> APLADYKDDDDKLAGTPSVDHGFLVTRHSQTIDDPQCPSGTKILYHGYSLLYVQGNERAHGQDLGTAGSCLRKFSTMPFLFCNINNVCNFASRNDYSYWLSTPEPMPMSMAPITGENIRPFISRCAVCEAPAMVMAVHSQTIQIPPCPSGWSSLWIGYSFVMHTSAGAEGSGQALASPGSCLEEFRSAPFIECHGRGTCNYYANAYSFWLATIERSEMFKKPTPSTLKAGELRTHVSRCQVCMGTGYLLVKHSQTDQEPMCPVGMNKLWSGYSLLYFEGQEKAHNQDLGLAGSCLARFSTMPFLYCNPGDVCYYASRNDKSYWLSTTAPLPMMPVAEDEIKPYISRCSVCEAPAIAIAVHSQDVSIPHCPAGWRSLWIGYSFLMHTAAGDEGGGQSLVSPGSCLEDFRATPFIECNGGRGTCHYYANKYSFWLTTIPEQSFQGSPSADTLKAGLIRTHISRCQVCMAPGFLVTRHSQTIDDPQCPSGTKILYHGYSLLYVQGNERAHGQDLGTAGSCLRKFSTMPFLFCNINNVCNFASRNDYSYWLSTPEPMPMSMAPITGENIRPFISRCAVCEAPAMVMAVHSQTIQIPPCPSGWSSLWIGYSFVMHTSAGAEGSGQALASPGSCLEEFRSAPFIECHGRGTCNYYANAYSFWLATIERSEMFKKPTPSTLKAGELRTHVSRCQVCMRRT

BMs are assembled from a toolkit of proteins that includes a collagen IV scaffold as a principal component. This scaffold confers structural integrity to tissues, binds integrins for cell adhesion and signaling, binds bone morphogenic proteins for signaling gradients during tissue development, and tethers a diverse assortment of molecules, including laminins, proteoglycans, and growth factors, which harbor a plethora of functions. Second, two protomers oligomerize via their trimeric noncollagenous (NC1) domains forming an NC1 hexamer at the junction, and four protomers oligomerize via the 7S domain forming a tetrameric structure. In protomer oligomerization, the interaction between trimeric NC1 domains is a chloride-dependent event.

Thus, native C41–C42 connections can be supplemented with similar artificial connections between C42 and C41 of adjacent domains to generate a single-chain α121 NC1 trimer (sc121 NC1 trimer) combining six C4 sub-domains. To determine the number and positions of Cl− ions involved into stabilization of the NC1 hexamer, here we purposely purified and crystallized the sc121 NC1-trimer in the presence of high chloride concentration to mimic natural extracellular Cl− content. Ultimately, it was crystallized in space group P41212 with a single polypeptide chain per asymmetric unit. Here, the hexamer is formed by two sc121 NC1-trimers related by a crystal 2-fold rotation symmetry. The overall atomic structure is identical to the previously reported structures for human and bovine NC1 domains isolated from tissues. All C4–C4 linkers, native and artificial, are well-structured and are related by a pseudo-hexagonal symmetry. Analysis of the hexamer formed from sc121 NC1-trimers revealed a set of 12 Cl− ions at the trimer–trimer interface. Collectively, all 12 Cl− at the trimer–trimer interface have well-defined and comparable electron density and B-factor values in the range from 23 to 27 Å2, like atoms of nearby residues. Together, the 12 ions form a chloride ring at the hexamer interface. Analysis of the solvent-accessible surface of the trimer and the hexamer shows that group 1 chloride ions are solvent-accessible in the trimer only, but group 2 ions remain solvent-exposed in the assembled hexamer. Group 1 ions induce hexamer assembly, and group 2 ions stabilize the hexamer structure.> SLLRQCPLLLPQNREGTAYEG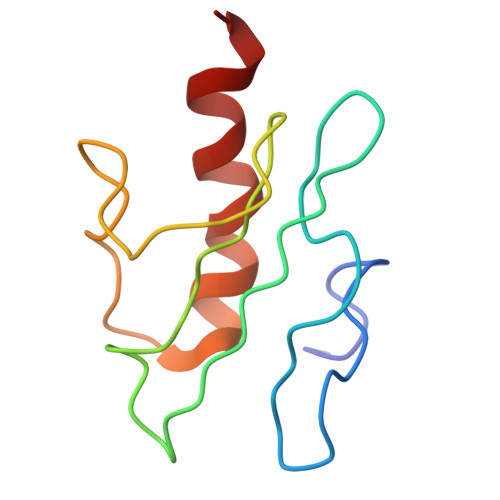FVSAQGRDFHIRILLPTDSQLKNARIECSWHLKKILHGYQHILKQRLHSCPDLVSFVVELKTILEIALKA>LMGCVAETPPRFTRTPVDQTGVSGGVASFICQATGDPRPKIVWNKKGKKVSNQRFEVIEFDDGSGSVLRIQPLRTPRDEAIYECVASNNVGEISVSTRLTVLREDQIPRGFPTIDMGPQLKVVERTRTATMLCAASGNPDPEITWFKDFLPVDTSNNNGRIKQLRSESIGGTPIRGALQIEQSEESDQGKYECVATNSAGTRYSAPANLYVRELREVRRVPPRFSIPPTNHEIMPGGSVNITCVAVGSPMPYVKWMLGAEDLTPEDDMPIGRNVLELNDVRQSANYTCVAMSTLGVIEAIAQITVKALPKPPGTPVVTESTATSITLTWDSGNPEPVSYYIIQHKPKNSEEPYKEIDGIATTRYSVAGLSPYSD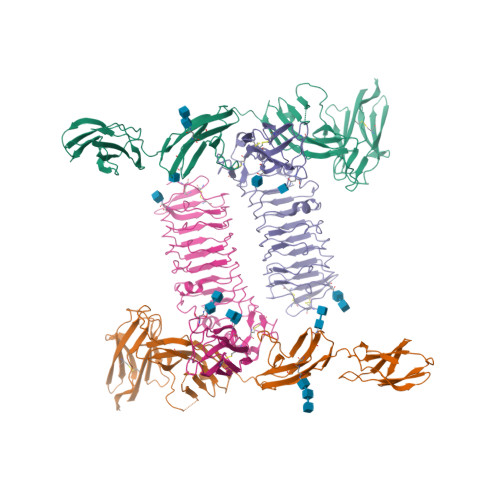YEFRVVAVNNIGRGPASEPVLTHHHHHH[2x];>QICPKRCVCQILSPNLATLCAKKGLLFVPPNIDRRTVELRLADNFVTNIKRKDFANMTSLVDLTLSRNTISFITPHAFADLRNLRALHLNSNRLTKITNDMFSGLSNLHHLILNNNQLTLISSTAFDDVFALEELDLSYNNLETIPWDAVEKMVSLHTLSLDHNMIDNIPKGTFSHLHKMTRLDVTSNKLQKLPPDPLFQRAQVLATSGIISPSTFALSFGGNPLHCNCELLWLRRLSREDDLETCASPPLLTGRYFWSIPEEEFLCEPPLITRHTHEMRVLEGQRATLRCKARGDPEPAIHWISPEGKLISNATRSLVYDNGTLDILITTVKDTGAFTCIASNPAGEATQIVDLHIIKLPHHHHHH[2x]> MTSTSIPTFPFDRPVPTEPSPMLSELRNSCPVAPIELPSGHTAWLVTRFDDVKGVLSDKRFSCRAAAHPSSPPFVPFVQLCPSLLSIDGPQHTAARRLLAQGLNPGFIARMRPVVQQIVDNALDDLAAAEPPVDFQEIVSVPIGEQLMAKLLGVEPKTVHELAAHVDAAMSVCEIGDEEVSRRWSALCTMVIDILHRKLAEPGDDLLSTIAQANRQQSTMTDEQVVGMLLTVVIGGVDTPIAVITNGLASLLHHRDQYERLVEDPGRVARAVEEIVRFNPATEIEHLRVVTEDVVIAGTALSAGSPAFTSITSANRDSDQFLDPDEFDVERNPNEHIAFGYGPHACPASAYSRM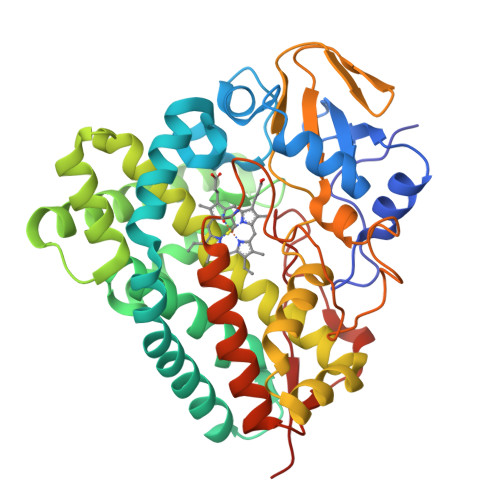CLTTFFTSLTQRFPQLQLARPFEDLERRGKGLHSVGIKELLVTWPT> SNAACGGGTTKESTANDATAAPSATTSAAADPNAPLKEGLKIAYLPKQLNNPYTDVEVGGGKVAVGEIKGEYKLVGPNDASASSQVSYINTLIQQQQDVIVVAANDPNAVCPSLNQARKADIKVVTFDSDAAKTCRDAFINQATTQGIGESLVKMAKELAGGSGEIAVL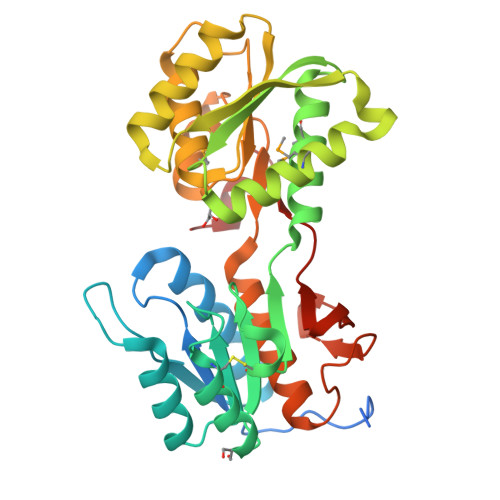SATPNATNQNSWIEVMKTELAKPENAKLKLVKIAYGNDDDQKSFTEAQGLLQSYPNLKVIVSPTTVGIAAASRYVSASSYKGKVAITGLGLPNQMRQYVKDGTVKKFALWNPADIGYLAAYAGAALKSGQITGAQGEKFKAGKLGEYTVGAAGEIVLGPPTEFTAANIDQFNF> 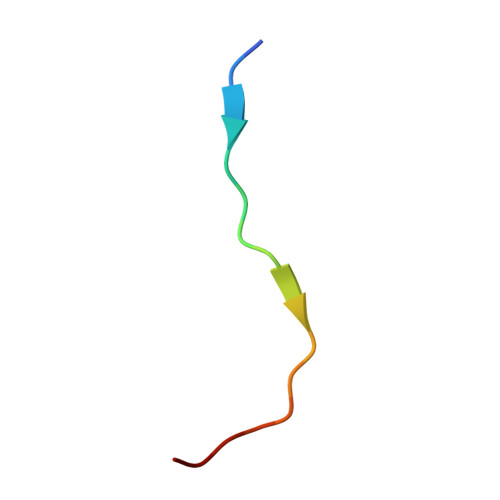RKQLMTKAARKSAPATG>MGSKYSKATNSINDALSSSYLVPFESYRVPLVDLEEATNNFDHKFLIGHGVFGKVYKGVLRDGAKVALKRRTPESSQGIEEFETEIETLSFCRHPHLVSLIGFCDERNEMILIYKYMENGNLKRHLYGSDLPTMSMSWEQRLEICIGAARGLHYLHTRAIIHRDVKSINILLDENFVPKITDFGISKKGTELGQTHLSTVVKGTLGYIDPEYFIKGRLTEKSDVYSFGVVLFEVLCARSAIVQSLPREMVNLAEWAVESHNNGQLEQIVDPNLADKIRPESLRKFGDTAVKCLALSSEDRPS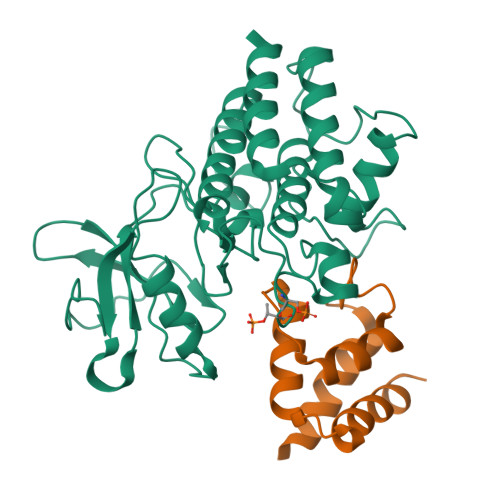MGDVLWKLEYALRLQESVIHHHHHH[4x];>[4x]PRRGAVAHANSIVQQLVSEGADISHTRNMLRNAMNGDAVAFSRVEQNIFRQHFPNMPMHGISRDSELAIELRGALRRAVHQQAAS> GSMSDGDYDYLIKFLALGDSGVGKTSVLYQYTDGKFNSKFITTVGIDFREKRVVYRANGPD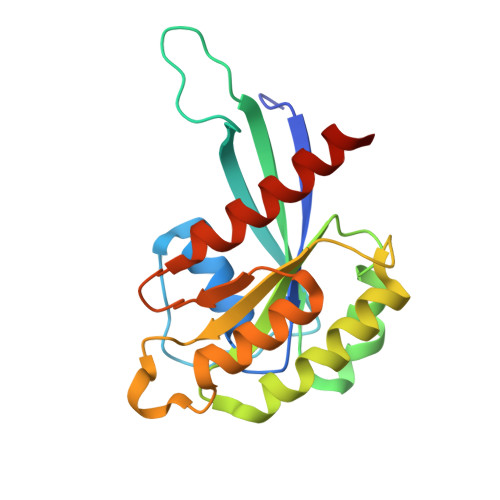GAVGRGQRIHLQLWDTAGLERFRSLTTAFFRDAMGFLLLFDLTNEQSFLNVRNWISQLQMHAYSENPDIVLCGNKSDLEDQRAVKEEEARELAEKYGIPYFETSAANGTNISHAIEMLLDLIMKRMERSVDKSW> SPTVEECGYSDRARSITLGNSTITTQECANVVVGYGVWPDYLKD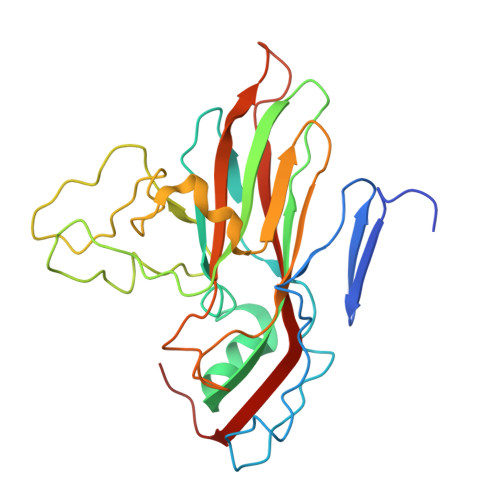SEATAEDQPTQPDVATCRFYTLDSVQWQKTSPGWWWKLPDALSNLGLFGQNMQYHYLGRTGYTVHVQCNASKFHQGCLLVVCVPEAEMGCATLDNTPSSAELLGGDTAKEFADKPVASGSNKLVQRVVYNAGMGVGVGNLTIFPHQWINLRTNNSATIVMPYTNSVPMDNMFRHNNVTLMVIPFVPLDYCPGSTTYVPITVTIAPMCAEYNGLRLAGHQ> INIGNKTNENVISFFDSTDAETQNHDVLMKGCGEFIVNLRTLLRTFRTITDNWILQANTKTPITDLTNTTDAQGRDYMSYLSYLYRFYRGGRRYKFFNTTPLKQ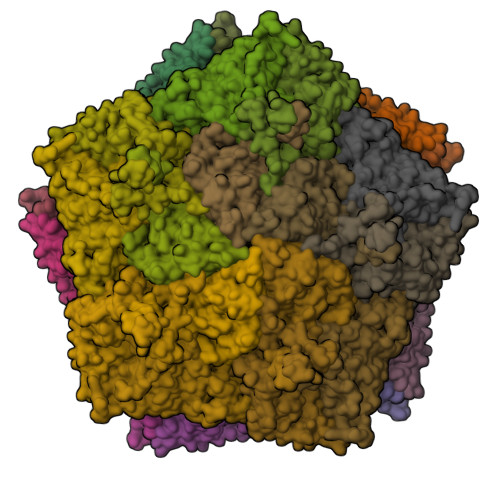SQTCYIRSFLMPRNYSADEINVDGPSHITYPVINPVHEVEVPFYSQYRKIPIASTSDKGYDSSLMYFSNTSTTQIVARAGNDDFTFGWMIGPPQLQGETRSVVP;> SKPRNQQQVCPLQNVPAWGYSLYKGIDMSVPLAYDPNNELGDLKDVFPSAVDEMAIGYVCGNPAVKHVLTWKTTDAIQKPIANGDDWGGVIPVGMPCYSKSIRTIKISETENRETEVIDAAPCEYVANMFSYWRATMCYRITVVKTAFHTGRLEIFFEPGVIPVKPTVNNIGPDQDQLTGAVAPSDNNYKYILDLTNDTEVTIRVPFVSNKMFLKTAGIYGANSENNWNFHESFSGFLCIRPVTKLMAPDTVSDNVSIVVWKWAEDVVVVEPKPLTSGPTQVYRPPPTASAAVEVLNVELQ;> DTHSIIQFLQRPVLIDNIEIIAGTTADAAKPLSRYVLDQQNSQKYVRSWTLPSTVLKAGGKAQKLANFKYLRCDVQVKLVLNANPFVAGRMYLAYSPYDDKVDTARSVLQTSRAGVTGYPGVELDFQLDNSVEMTIPYASFQEAYDLVTGTEDFVQLYLFPITPVLGPKSESESSKVDISVYMWLSNISLVIPTYRMNPD> ASMTTPCITILSGHFPKETIYARKTKELVEEYCSIHGYNFYYEESEPLETEEHALHFRRSWIIQQAAEKFPSTEWFLWLDSDVYVNPKNKNKPITSFIDLSDPNILYHTFHEAPWGSYPINTGVKFVHKDALEIEKIVWSLRNEAPWNTFPYEQKTV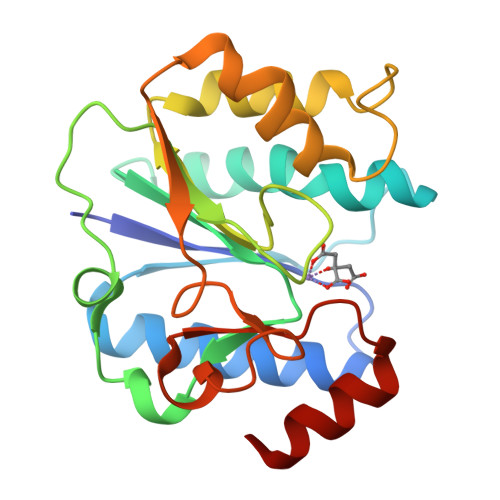YEYVFPRIPGRYIVHDPYTLNCIVKAYPEHVKDALFVHMCGTSRAERDEHMEMVAT O-benzyl-L-serine 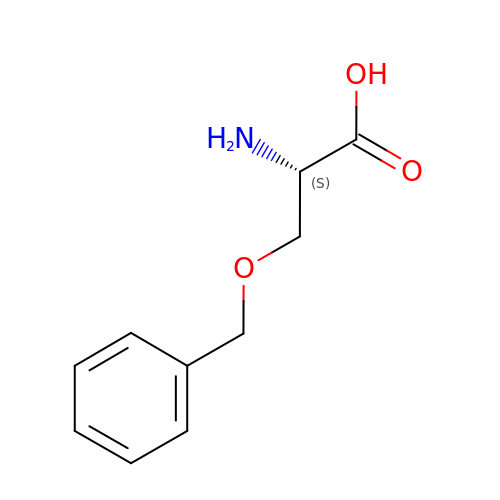| C10 H13 N O3 | IDGQXGPQOGUGIX-VIFPVBQESA-N>GGRVRTGQVPVSVNYHFSRKCNKECLFCFHTATTSHVEKPENAKRGLTLLKQAGMKKINFAGGEPFLYPKFLGEMIDFCKETLQLESVSIVTNGSLVKEQF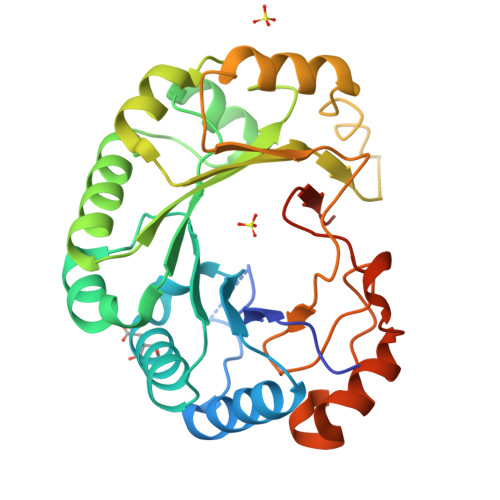LQKHGRNIDILAVSCDSFNEATNIKIGRGSGDNVQKLYEIGSWCQKYDIKFKLNTVVNKFNHLEDMNDHLNALQPFRWKCFQVLIVTGENDSDKTLRNAHSLTISDDEFDRFCERHSSQTCLVPEPNRLMAKSYLILDEYMRFLDRNGQQPSKSILEVGVQQALQAVFWDEEAFVERGGIYDWNKSSCSSDSKDLEW[12x]>MSSEFISKVDKEARRKAANILRDKFLNLVEQLKKGEPLVMEIPMRTLSNAIYDEKRKLLLLGEKKLRRNFLDLNEAKRFMQTVLMASIIYDALVSDEYPTIRDLYYRGKHSLLLKSIEGNKIVSEENTWDEQKESDSVIVDIEVFTSLLREEMLILSKEKGKVVGNLRIRSGNDVIDLSKTGHGAYAIEPTPDLIDFIDVDAEFVLVVEKDAVFQQLHRAGFWKQYKSILITSAGQPDRATRRFVRRLNEELKLPVYILTDADPYGWYIFSVFRIGSISLSYESERLATPDAKFLGVSMGDIFGNSRKKPYLSEAERKNYIIKAKDADIKRAEEIKNYEWFKTKAWQEEINTFLQRKAKLEIEAMASKGLKFLAFQYIPEKITNKDYIA[4x];>[4x]MSAKEKFTSLSPAEFFKRNPELAGFPNPARALYQTVRELIENSLDATDVHGILPNIKITIDLIDDARQIYKVNVVDNGIGIPPQEVPNAFGRVLY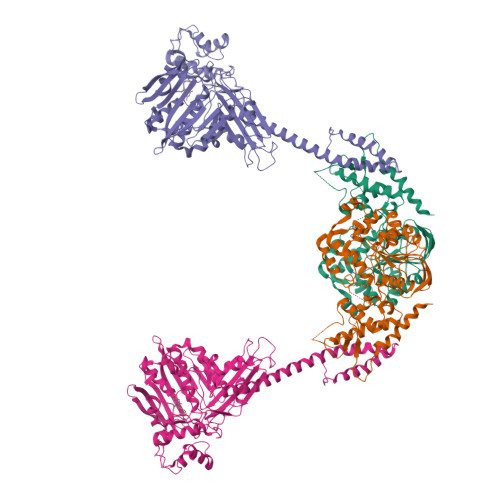SSKYVNRQTRGMYGLGVKAAVLYSQMHQDKPIEIETSPVNSKRIYTFKLKIDINKNEPIIVERGSVENTRGFHGTSVAISIPGDWPKAKSRIYEYIKRTYIITPYAEFIFKDPEGNVTYYPRLTNKIPKPPQEVKPHPYGVDREEIKILINNLKRDYTIKEFLVNEFQSIGDTTADKILELAGLKPNKKVKNLTEEEITRLVETFKKDEDFRSPSADSLSVIGEDLIELGLKKIFNPDFAASITRKPKAYQGHPFIVEAGVAFGGSIPVGEEPIVLRYANKIPLIYDEKSDVIWKVVEELDWKRYGIESDQYQMVVMVHLCSTKIPYKSAGKESIAEVENIEKEIKNALMEVARKLKQYLSEKRKEQEAKKKLLAYLKYIPEVSRSLATFLASGNKELVSKYQNEISEGLFKLISKKLDLINIEEYRKVYRVDSE N-Ethyl 4-((1-cycloheptyl-1,2-dihydropyrazol-3-one-5-yl)-amino)-4-oxo-butanamide | C16 H26 N4 O3 | 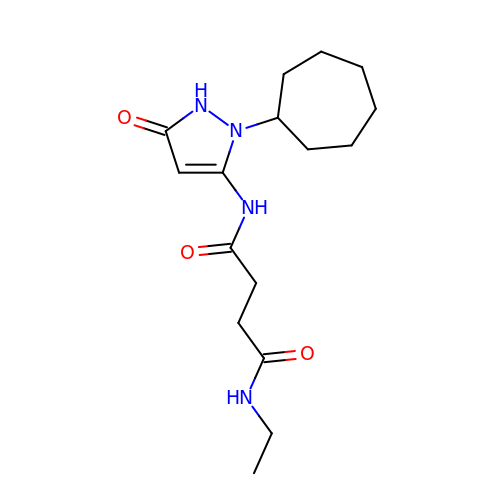LPNCMHPJRSJOIM-UHFFFAOYSA-N> MKKVVAVVKLQLPAGKATPAPPVGPALGQHGANIMEFVKAFNAATANMGDAIVPVEITIYADRSFTFVTKTPPASYLIRKAAGLEKGAHKPGREKVGRITWEQVLEIAKQKMPDLNTTDLEAAAR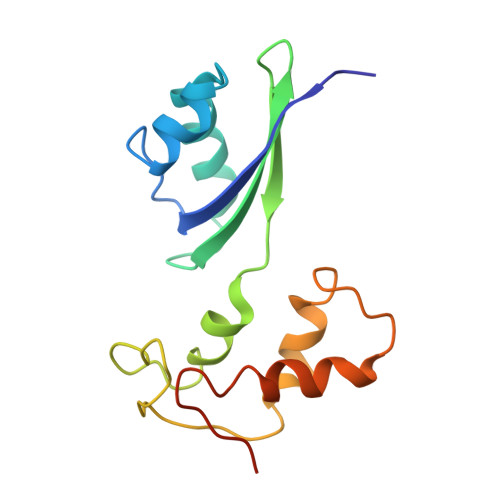MIAGSARSMGVEVVGAPEVKDA>[2x]MANVSKKVSWSGRDRDDEEAAPLLRRTARPGGGTPLLNGAGPGAARQSPRSALFRVGHMSSVELDDELLDPDMDPPHPFPKEIPHNEKLLSLKYESLDYDNSENQLFLEEERRINHTAFRTVEIKRWVICALIGILTGLVACFIDIVVENLAGLKYRVIKGNIDKFTEKGGLSFSLLLWATLNAAFVLVGSVIVAFIEPVAAGSGIPQIKCFLNGVKIPHVVRLKTLVIKVSGVILSVVGGLAVGKEGPMIHSGSVIAAGISQGRSTSLKRDFKIFEYFRRDTEKRDFVSAGAAAGVSAAFGAPVGGVLFSLEEGASFWNQFLTWRIFFASMISTFTLNFVLSIYHGNMWDLSSPGLINFGRFDSEKMAYTIHEIPVFIAMGVVGGVLGAVFNALNYWLTMFRIRYIHRPCLQVIEAVLVAAVTATVAFVLIYSSRDCQPLQGGSMSYPLQLFCADGEYNSMAAAFFNTPEKSVVSLFHDPPGSYNPLTLGLFTLVYFFLACWTYGLTVSAGVFIPSLLIGAAWGRLFGISLSYLTGAAIWADPGKYALMGAAAQLGGIVRMTLSLTVIMMEATSNVTYGFPIMLVLMTAKIVGDVFIEGLYDMHIQLQSVPFLHWEAPVTSHSLTAREVMSTPVTCLRRREKVGVIVDVLSDTASNHNGFPVVEHADDTQPARLQGLILRSQLIVLLKHKVFVERSNLGLVQRRLRLKDFRDAYPRFPPI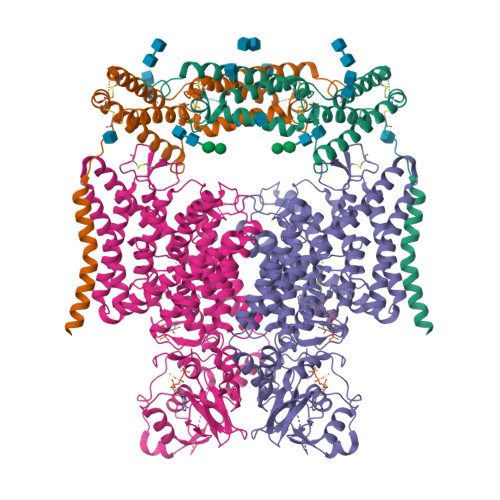QSIHVSQDERECTMDLSEFMNPSPYTVPQEASLPRVFKLFRALGLRHLVVVDNRNQVVGLVTRKDLARYRLGKRGLEELSLAQT;>MEPGPTAAQRRCSLPPWLPLGLLLWSGLALGALPFGSSPHRVFHDLLSEQQLLEVEDLSLSLLQGGGLGPLSLPPDLPDLDPECRELLLDFANSSAELTGCLVRSARPVRLCQTCYPLFQQVVSKMDNISRAAGNTSESQSCARSLLMADRMQIVVILSEFFNTTWQEANCANCLTNNSEELSNSTVYFLNLFNHTLTCFEHNLQGNAHSLLQTKNYSEVCKNCREAYKTLSSLYSEMQKMNELENKAEPGTHLCIDVEDAMNITRKLWSRTFNCSVPCSDTVPVIAVSVFILFLPVVFYLSSFLHSEQKKRKLILPKRLKSSTSFANIQENSN[2x]>MHHHHHHMANCERTFIAIKPDGVQRGLV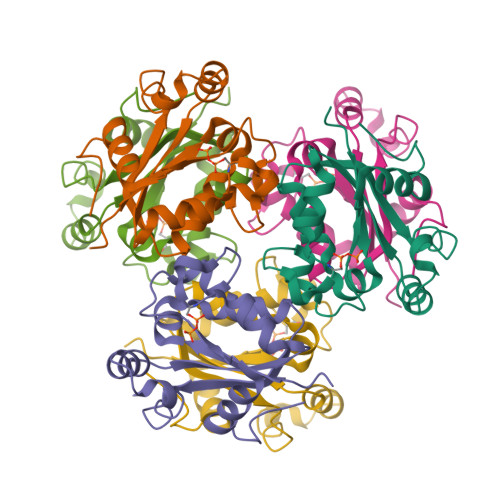GEIIKRFEQKGFRLVGLKFMQASEDLLKEHYVDLKDRPFFAGLVKYMHSGPVVAMVWEGLNVVKTGRVMLGESNPADSKPGTIRGDFCIQVGRNIIHGSDSVESAEKEIGLWFHPEELVDYTSCAQNWIYE[6x]>[2x]HHHHHMIVLFVDFDYFYAQVEEVLNPSLKGKPVVVCVFSGRFEDSGAVATANYEARKFGVKAGIPIVEAKKILPNAVYLPMRKEVYQQVSSRIMNLLREYSEKIEIASIDEAYLDISDKVRDYREAYNLGLEIKNKILEKEKITVTVGISKNKVFAKIAADMAKPNGIKVIDDEEVKRLIRELDIADVPGIGNITAEKLKKLGINKLVDTLSIEFDKLKGMIGEAKAKYL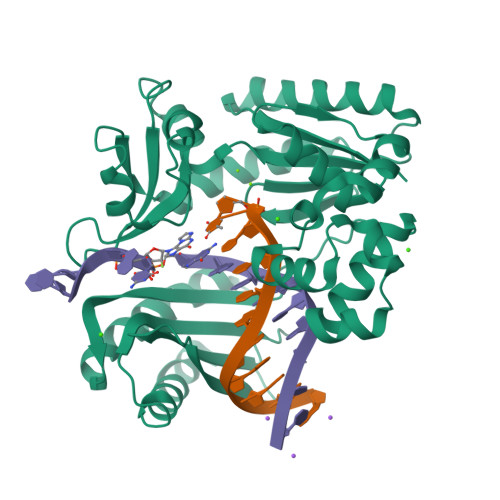ISLARDEYNEPIRTRVRKSIGRIVTMKRNSRNLEEIKPYLFRAIEESYYKLDKRIPKAIHVVAVTEDLDIVSRGRTFPHGISKETAYSESVKLLQKILEEDERKIRRIGVRFSKFIE> MRRINFNDNWRFQREISTSLREAQKPSFNDHSWRQLSLPHDWSIELDFNKDSLATHEGGYLDGGVGWYRKTFTVPSAMEGKRISLDFDGVYMNSTTYLNGEELGTYPFGYNAFSYDITDKLFMDGRENVLAVKVDNTQPSSRWYSGSGIYRNVYLTVTNPVHVARYGTFVTTPDLESAYAARKAEVNIKTKINNDSDAAVQVKVKSTIYDTD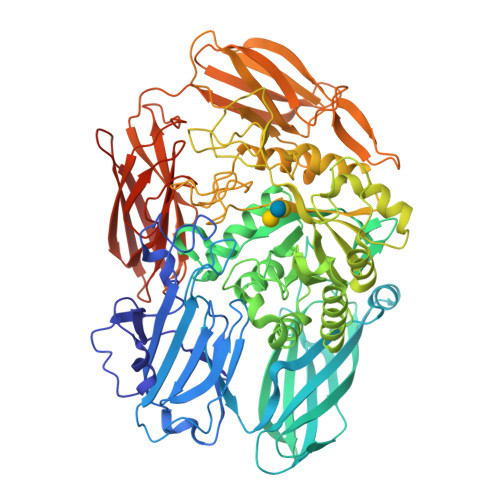GKEVASVVSQEKTAAAGTTAHFEDNTVIENPELWSLDNPYRYKLVTDVLIGGETVDTYETRFGARFFKFDANEGFSLNGKPMKLYGVSMHHDLGALGAATNARAVERQLQIMKDMGVNAIRGTHNPVSPEFLEAVNNLGLLLIEEAFDCWSQSKKTYDYGRFFTRWAEHDVKEMVDRGKNEPSIIMWSIGNEIYDTTSPSGVETARNLVRWIKEIDTTRPTTIGEDKTRGDKVNVTPIDPNILEIFHTVDVVGLNYSENNYVGYHEQHPNWKLYGSETSSATRSRGVYTHPYEYNLGTKYDDLQQSSYDNDYVPWGRTAEDAWKSDRDLKHFAGQFIWTGFDYIGEPTPYYDSYPAKSSYFGAVDTAGFPKDIFYYYQSQWKKEPMVHLLPHWNWTEGEPVRVLAYTNAHQVELFLNGKSLGVRGYENKKTSWGAPYKETKDGKTYLEWAVPFKAGTLEAVAMDENGKEIARDQVTTAGAPAAVKLTADRKVIKADGTDLSFITAEIVDSKGNVVPNADHLIQFHLSGHGELAGVDNGDAASVERYKDNKRKAFSGKALAIVQSNKLDGNITLHASAEGLSSGNVTIFTTASADQLEHHHHHH> CLAEGTRIFDPVTGTTHRI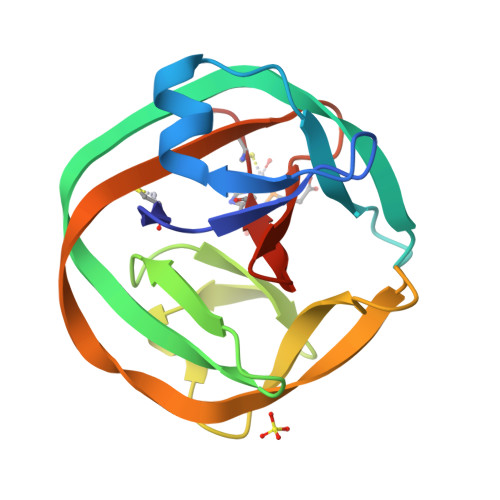EDVVDGRKPIHVVAAAKDGTLHARPVVSWFDQGTRDVIGLRIAGGAILWATPDHKVLTEYGWRAAGELRKGDRVAVRDVETGELRYSVIREVLPTRRARTFDLEVEELHTLVAEGVVVHACSPPF> MSAEKLFTP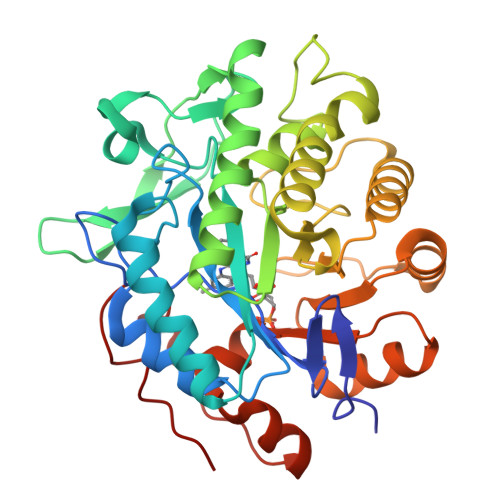LKVGAVTAPNRVFMAPLTRLRSIEPGDIPTPLMGEYYRQRASAGLIISEATQISAQAKGYAGAPGLHSPEQIAAWKKITAGVHAEDGRIAVQLWHTGRISHSSIQPGGQAPVSASALNANTRTSLRDENGNAIRVDTTTPRALELDEIPGIVNDFRQAVANAREAGFDLVELHSAHGYLLHQFLSPSSNQRTDQYGGSVENRARLVLEVVDAVCNEWSADRIGIRVSPIGTFQNVDNGPNEEADALYLIEELAKRGIAYLHMSETDLAGGKPYSEAFRQKVRERFHGVIIGAGAYTAEKAEDLIGKGLIDAVAFGRDYIANPDLVARLQKKAELNPQRPESFSGGGAEGYTDYPSL> GKEKHKI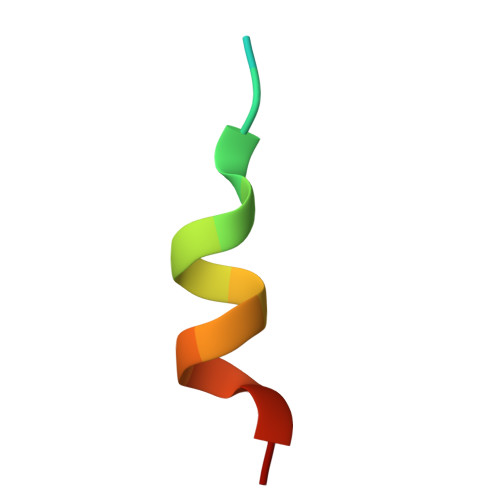LHRLLQDSS> ADGKYAQKLFNDLFEDYSNALRPVEDTDKVLNVTLQITLSQIKDMDERNQILTAYLWIRQIWHDAYLTWDRDQYDGLDSIRIPSDLVWRPDIVLYNKADDESSEPVNTNVVLRYDGLITWDAPAITKSSCVVDVTYFPFDNQQCNLTFGSWTYNGNQVDIFNAL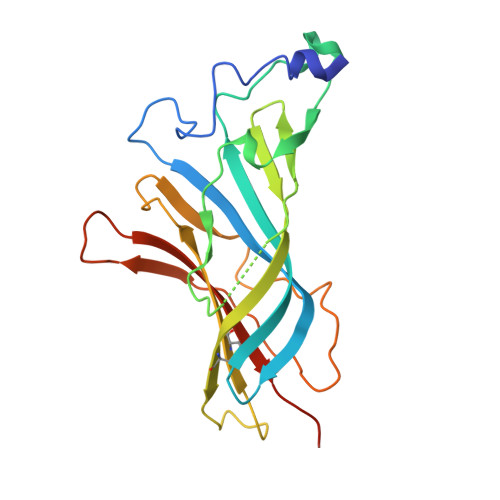DSGDLSDFIEDVEWEVHGMPAVKNVISYGCCSEPYPDVTFTLLLKRRSHHHHHH> MGSDKIHHHHHHENLYFQGMNIETLMIKNPPILSKEDRLGSAFKKINEGGIGRIIVANEKIEGLLTTRDLLSTVESYCKDSCSQGDLYHISTTPIIDYMTPNPVTVYNTSDEFTAINIMVTRNFGSLPVVDINDKPVGIVTEREFLLLYKDLDEIFPVKVFMSTKVQTIYKEVRLDQAVKLMLRRGFRRLPVIDDDNKVVGIVTVVNAIKQLAKAVDKLDPDYFYGKVVKDVMVTNLVTIDELASVNRAAAEMIVKRI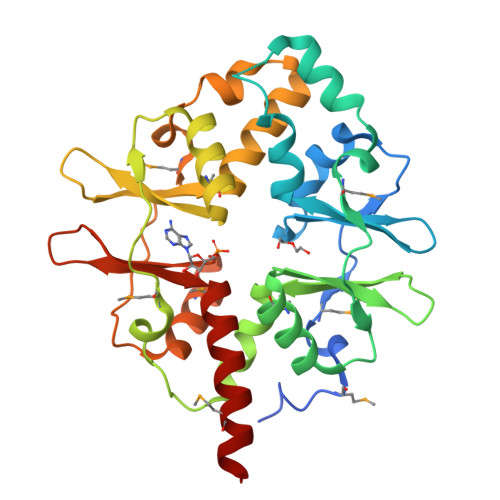GSLLILNKDNTIRGIITERDLLIALHHILVMEKFKEKL>[28x]SNATAYIIVGLTPKDAEKLQQYGARVAS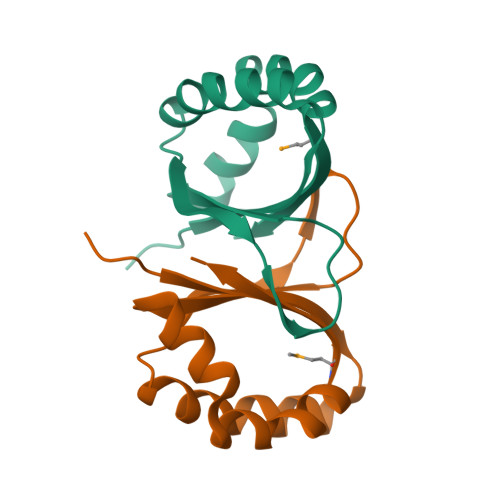TLAKYSGEVLVKGSVEQLHGKFEHKAQVILEFPSREDAYNWYHSEEYQALISTRDLGMDSQFQLIG Nonstructural protein 3 (nsp3), an essential component of the replication/transcription complex, is one of the most important antiviral targets. Nsp3 is essential for the formation of the RTC, and it functions as a scaffold protein by interacting with itself and other proteins (including viral nsps and host proteins). Affinity for adenosine diphosphate ribose (ADPr) or poly-ADP-ribose is a well-known characteristic of Macro, and in some cases, it also shows ADP-ribose 1″-monophosphatase (ADRP) activity; however, the biological significance of this enzyme activity remains unclear. PLpro is responsible for the hydrolytic release of nsp1/2 -nsp4; in addition to hydrolytic activity, PLpro also possesses deubiquitinating and deISGylating activities.

Here, we first report the structure of PDCoV Macro-Ubl2-PLpro from δ-CoV with 2.5 Å resolution. The Macro-Ubl2-PLpro monomer consists of three distinct domains: Macro, Ubl2, and PLpro. At the flanking N-terminus of the crystal structure, Macro adopts a conserved three-layered α-β-α sandwich fold, similar to the macroH2A variant of human histone 2A. Amino acids (aa 166-215) fold into a ubiquitin-like 2 domain, which lies in front of PLpro and is well separated from PLpro and Macro. The thumb, palm and finger domains form the catalytic core of PLpro, which has an extended right-hand architecture. At the tip of the finger domain, four cysteines (Cys334, Cys335, Cys360 and Cys363) from two β-hairpins that coordinate a zinc ion with a tetrahedral structure. The short BL2 in PDCoV PLpro causes the space for substrate binding to be much larger than the corresponding spaces of USP14 and other CoV PLPs. We determined that the active sites of PDCoV PLpro consist of Cys and His residues, similar to the active sites observed in many PLPs. Cys260 is located at the base of α9 of the thumb 3.6 Å from His398, which is situated at the base of the palm domain, while the third hypothetically conserved site aspartic acid (Asp412) is not well aligned with Cys260 and His298, the position of PDCoV PLpro Asp412 is quite inconsistent among other PLPs, and the possible explanation is that the Asp412 is located on the flexible loop connecting β19 and β20 (Figure 3(A) and Figure 6(A–C)). In the asymmetric unit, two of the subunits form the head-to-tail homodimer, with a total area of 807.3 Å2 buried in the interface. The SAXS profile calculated based on the monomer crystal structure is consistent with that in solution, while the profile calculated based on the dimer crystal structure is inconsistent, indicating that the protein is monomer in solution.

> LPPEAIKQPSPTKVELVVGELASIKFDNSVLVNPANAQLTNGGGAARAIAKLAGPKYQEYCNSVAPISGPLTTDSFDAKKLGVACILHVVPPKGSDPNVQELLYQAYKSILTEPAHYVIPILGAGIFGCNPVHSLDAFRKACPSDIGRVTLVTMNKNHLQVWDALNRTIVRTTTDYDQVTTKALTPQGVLEANLFDGEDFVQEPKPGQIYLEVTEEVQNQAKELDLNLQQYCVYLKTCHHKWVVSRTNGLMHLKQKDNNCFVSAGVNLFQNTAYQFRPAIDALYREYLNGNPNRFVAWIYASTNRRVGEMGCPQQVISLLVSNSDAAFSATTACCNTYFNHTGVISVAREYDPIQPKVYCMKCDVWTPFTPQSGKGAVAIGTSADEPTGPAIKFAAAHCWYTNGKKTVNGYDTKANVVATYHRFDVPKPQLVEDVVALPTKNDFEHHHHHH4'-DEOXY-4'-IODODOXORUBICIN | C27 H29 I N O10 | 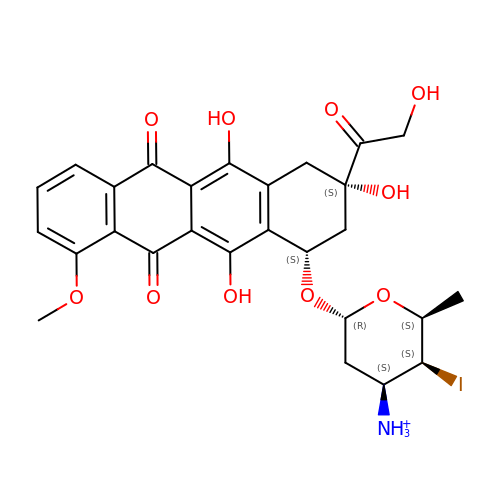PDQGEKGUTOTUNV-TZSSRYMLSA-O> FPTDDDDKIVGGYTCAANSIPYQVSLNSGSHFCGGSLINSQWVVSAAHCYKSRIQVRLGEHNIDVLEGNEQFINAAKIITHPNFNGNTLDNDIMLIKLSSPATLNSRVATVS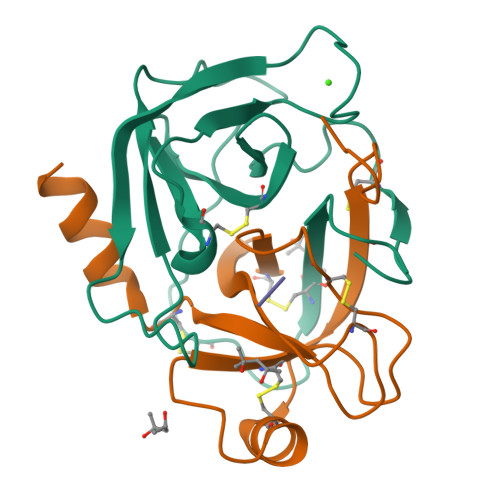LPRSCAAAGTECLISGWGNTK;> SSGSSYPSLLQCLKAPVLSDSSCKSSYPGQITGNMICVGFLEGGKDSCQGDSGGPVVCNGQLQGIVSWGYGCAQKNKPGVYTKVCNYVNWIQQTIAAN Modulation of voltage-gated potassium (Kv) channels by auxiliary subunits is central to the physiological function of channels in the brain and heart. Native Kv4 tetrameric channels form macromolecular ternary complexes with two auxiliary β-subunits—intracellular Kv channel-interacting proteins (KChIPs) and transmembrane dipeptidyl peptidase-related proteins (DPPs)—to evoke rapidly activating and inactivating A-type currents, which prevent the backpropagation of action potentials. Here we report cryo-electron microscopy structures of the Kv4.2–DPP6S–KChIP1 dodecamer complex, the Kv4.2–KChIP1 and Kv4.2–DPP6S octamer complexes, and Kv4.2 alone. Thus, our data suggest that two distinct modes of modulation contribute in an additive manner to evoke A-type currents from the native Kv4 macromolecular complex.

KChIP1s are laterally anchored next to the T1 domains of Kv4.2, consistent with the previous crystal structures of the Kv4.3 T1 domain–KChIP1 complex. The N-terminal hydrophobic segment (A2–R35) of Kv4.2, referred to as the inactivation ball, was captured by KChIP1, which may explain why Kv4.2 exhibits a closed inactivated (CSI) mechanism, rather than an open inactivated (OSI) mechanism like Kv1.2, as previously discussed for Kv4.326,27. Although the residues from G451 to G471 are disordered, the following second cytoplasmic helix with a short loop (C-terminal segment: S472–D495) fits into the hydrophobic crevice formed by KChIP1 and the Kv4.2 N-terminal segment (A2–R35) from the neighbouring Kv4.2 subunit. In addition, the cytoplasmic S6 helix (around S450) is captured by KChIP1 directly and indirectly, through the hydrophobic interactions between Kv4.2 (Y444), Kv4.2 (H479-L482-F493) and KChIP1 (H84) and the electrostatic interactions of Kv4.2 (Y444–K448) with Kv4.2 (H483–E486), respectively. The amino acid sequence of the C-terminal helix segment (S473–T489) perfectly matches the dendritic targeting motif that is conserved in the Shal family of potassium channels—including Kv4—suggesting that this motif has a dual function as a KChIP-binding site and a dendrite localization signal. In the Kv4.2–KChIP1 complex, KChIP1s bind and sequester the both N-terminal inactivation ball and the C terminus (amino acids 472–495) of Kv4.2, which would therefore result in preventing N-type inactivation.

>[4x]AAGVAAWLPFARAAAIGWMPVASGPMPAPPRQERKRTQDALIVLNVSGTRFQTWQDTLERYPDTLLGSSERDFFYHPETQQYFFDRDPDIFRHILNFYRTGKLHYPRHECISAYDEELAFFGLIPEIIGDCCYEEYKDRRRENAERLQDDADTDTAGESALPTMTARQRVWRAFENPHTSTMALVFYYVTGFFIAVSVIANVVETVPCGSSPGHIKELPCGERYAVAFFCLDTACVMIFTVEYLLRLAAAPSRYRFVRSVMSIIDVVAILPYYIGLVMTDNEDVSGAFVTLRVFRVFRIFKFSRHSQGLRILGYTLKSCASELGFLLFSLTMAIIIFATVMFYAEKGSSASKFTSIPAAFWYTIVTMTTLGYGDMVPKTIAGKIFGSICSLSGVLVIALPVPVIVSNFSRIYHQNQRADKRRAQKKARLARIRAAKSGSANAYMQSKRSGLLSNQLQSSEDEQAFVSKSGSSFETQHHHLLHCLEKTTNHEFVD;>[4x]PEGLEQLEAQTNFTKRELQVLYRGFKNECPSGVVNEDTFKQIYAQFFPHGDASTYAHYLFNAFDTTQTGSVKFEDFVTALSILLRGTVHEKLRWTFNLYDINKDGYINKEEMMDIVKAIYDMMGKYTYPVLKEDTPRQHVDVFFQKMDKNKDGIVTLDEFLESCQEDDNIMRSLQLFQNVM>MTIVQAAQSRYSTKAFDASRKLPEEKVAAVKELIRMSASSVNSQPWHFIVASSEEGKARIAKATQGGFAANERKILDASHVVVFCAKTAIDEAYLLDLLESEDKDGRYADVEAKNGMHAGRSFFVNMHRFDLKDAHHWMEKQVYLNVGTLLLGASAMEIDAVPIEGFDAKVLDEEFGLREKGFTSVVIVPLGYHSEDDFNAKLPKSRWSAETVFTEI[2x]

Of particular interest are type I (oxygen independent) bacterial nitroreductases, which are flavoenzymes that catalyse the concerted transfer of two electrons from reduced nicotinamide adenine dinucleotide (phosphate) (NAD(P)H) to the nitro group of the substrate. This results in the formation of a reduced nitroso intermediate, which subsequently undergoes further reduction to generate the final hydroxylamine or amine product(s). Instead, active site amino acid residues act to stabilise the charge on the reduced form of the flavin mononucleotide (FMN) cofactor and form binding pockets that position the substrate, NADPH and FMN at optimal distances for efficient hydride transfer. Each dimer has two active sites, formed at this interface and comprised of residues from both monomers.

NTR 2.0 was derived from the NfsB orthologue of Vibrio vulnificus by introduction of rationally identified F70A and F108Y residue substitutions. To better understand the improved enzymatic mechanism of NTR 2.0, we have now crystallised and solved the structure of NTR 2.0 to 1.85 Angstrom resolution. The asymmetric unit contained two NTR 2.0 molecules, with a Matthews coefficient of 2.32 Å3/Da and a solvent content of 47%. The structure of NTR 2.0 is a homodimer, with each monomer composed of 14 α-helices and 4 β-sheets (with connecting turns and loops). In both our wild-type and mutant structures, one FMN and one acetate molecule occupy each active site. NTR 2.0 and the parental enzyme share high structural similarity (root-mean-square deviation (RMSD) of 0.32 Å); however, significant differences were noted in the active site. In the NTR 2.0 structure, mutation of active site residue 108 from phenylalanine to tyrosine introduces hydrogen bonding from the Y108 hydroxyl group to nearby residue E102. This new bond may stabilise the active site, lowering the energy of the transition state during metronidazole catalysis. Notably, the NTR 2.0 structure also exhibits a widened substrate entrance channel compared to the wild-type, resulting from the displacement of residues F123, F124 and F68 and the removal of the aromatic side chain at residue F70. Widening of this channel likely reduces steric hindrance, potentially allowing faster and more efficient passage of NAD(P)H cofactor, reactants and end-products into and out of the active site.> MEKLKEFLKGVRDELKRVVWPSRELVVKATI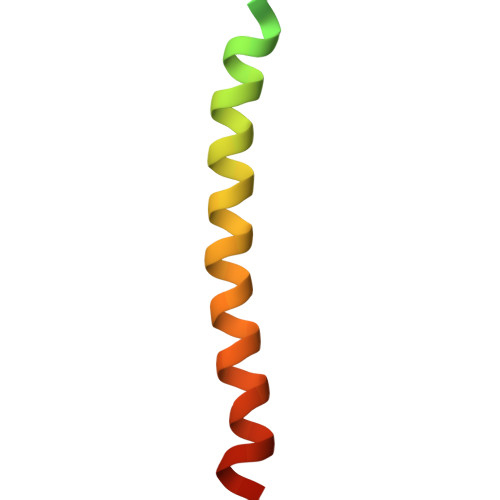SVIIFSLAIGVYLWILDLTFTKIISFILSLRGSL>MPPYTVVYFPVRGRCAALRMLLADQGQSWKEEVVTVETWQEGSLKASCLYGQLPKFQDGDLTLYQSNTILRHLGRTLGLYGKDQQEAALVDMVNDGVEDLRCKYISLIYTNYEAGKDDYVKAL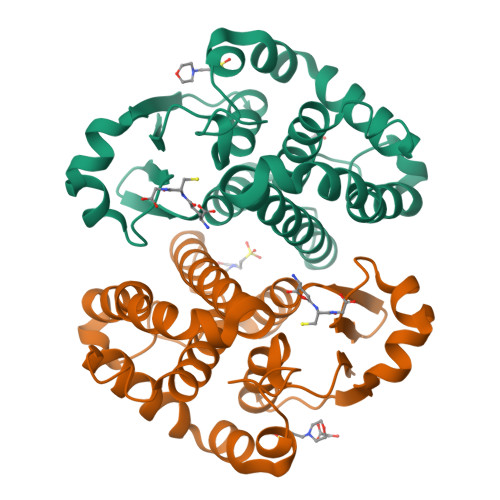PGQLKPFETLLSQNQGGKTFIVGDQISFADYNLLDLLLIHEVLAPGCLDAFPLLSAYVGRLSARPKLKAFLASPEYVNLPINGNGKQ[4x]>AEDGPQKQQLEMPLVLDQDLTQQMRLRVESLKQRGEKKQDGEKLIRPAESVYRLDFIQQQKLQFDHWNVVLDKPG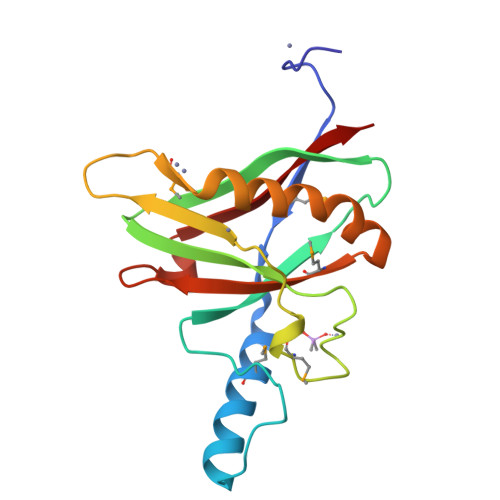KVTITGTSQNWTPDLTNLMTRQLLDPAAIFWRKEDSDAMDWNEADALEFGERLSDLAKIRKVMYFLITFGEGVEPANLKASVVFNQL[2x]5'-azido-5'-deoxy-8-[(2-{[2-(3-ethynylphenyl)ethyl]amino}-2-oxoethyl)sulfanyl]adenosine | C22 H23 N9 O4 S | 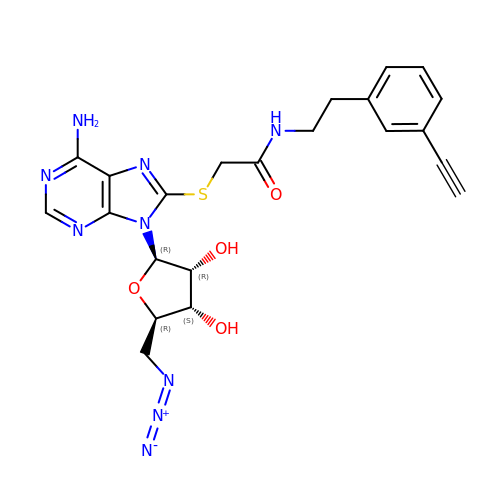HEZMFPGXYOAFRQ-HAXDFEGKSA-N>SMKIFNKESLNQLEKKGYLIIDNFLNDLNKINLIYDESYNQFKENKLIEAGMNKGTDKWKDKSIRGDYIQWIHRDSNSRIQDKDLSSTIRNINYLLDKLDLIKNEFDNVIPNFNSIKTQTQLAVYLNGGRYIKHRDSFYSSE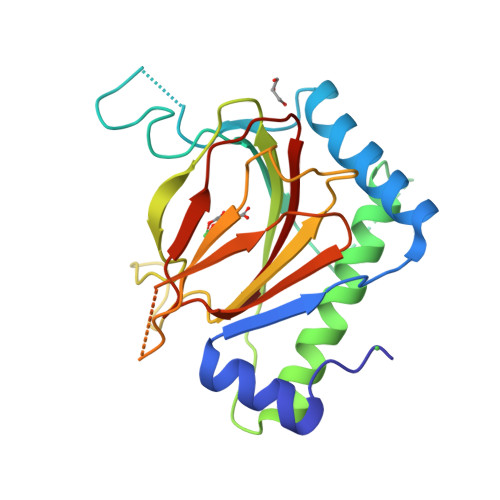SLTISRRITMIYYVNKDWKKGDGGELRLYTNNPNNTNQKELKQTEEFIDIEPIADRLLIFLSPFLEHEVLQCNFEPRIAITTWIY[3x]> GPHTVAEKQDTLVPAGPAKAVLEVNDELLKAVASGDWDAYTTMVDPNVTCFEPEAAGVLAKGLAFHKF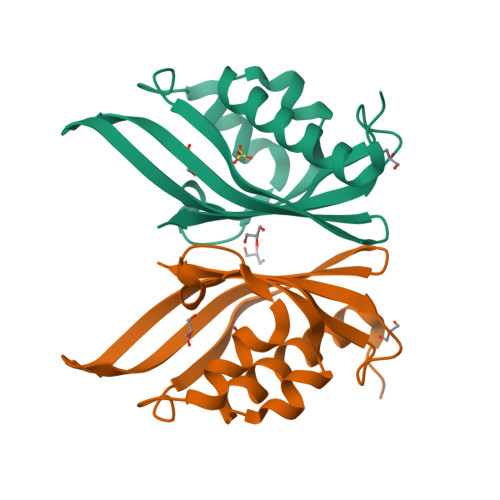FFDNRSPNADKMKTTLHDPAVQMFGDTAIVTALRVVQFVADDGPKTTRYEETRVWVKDAAFKFGWKLVHFHRSGAHATPN>MVLYFIGLGLYDERDITVKGLEIAKKCDYVFAEFYTSLMAGTTLGRIQKLIGKEIRVLSREDVELNFENIVLPLAKENDVAFLTPGDPLVATTHAELRIRAKRAGVESYVIHAPSIYSAVGITGLHIYKFGKSATVAYPEGNWFPTSYYDVIKENAERGLHTLLFLDIKAEKRMYMTANEAMELLLRVEDMKKGGVFTDDTLVVVLARAGSLNPTIRAGYVKDLIREDFGDPPHILIVPGKLHI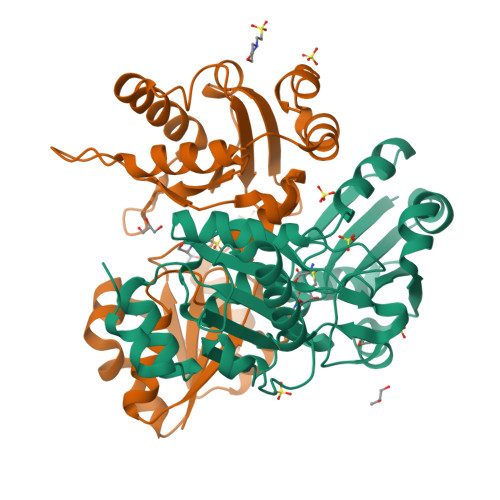VEAEYLVEIAGAPREILRVNV[2x]>GSAKDPMRVLKYAILGLLRKGELSGYDITSYFKEELGQFWSAKHSQIYPELKKLTDEGFITFRTTIQGTKLEKKMYTLTDSGKQELHDWLIRHQPIPETVKDEFMLKAYFISSLSRQEASDLFTDQLLKRKAKLSDLQGSYEKLMASAEPMSFSSPDFGHYLVLTKALEREKNYVSWLESILAM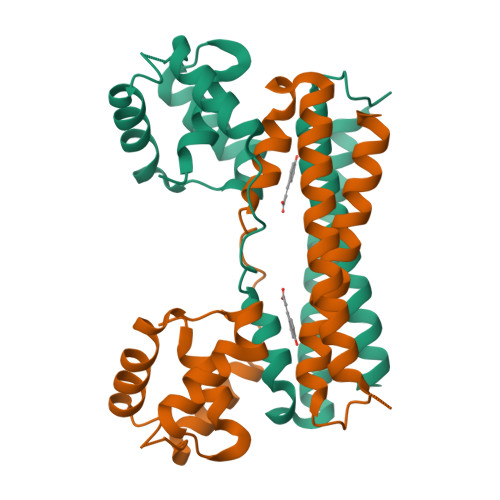IDED[3x]> HHHHHHMFDVAKYLRRIGVEGTPPPTLDTLRHLHKRHLMAVPYDNSTAPDRLPASRHLTNVPLDLVFGHVVTEGHGGVCYELNRLFHTLLAELGYDVRMVAAAVRQANGTFGPEREHTFDLVHLDGRTHLVDVGFPGPSYSEPLYLSEEEQHQYGCSYRVTEHDGYRVVERRPKGSDWQPVYRFRPELADPSGWDAVRLLDSLDDYAQDSVLGTTFRSRATDNGKIVLIGRRYFTVEDGVERTKVLVKADEFQDVVDLILAGA

Amide synthases catalyze the formation of macrolactam rings from aniline-containing polyketide-derived seco-acids as found in the important class of ansamycin antibiotics. A key enzyme is the amide synthase ShGdmF (hereafter abbreviated as GdmF), which is not part of the PKS and is thought to catalyze the release of the ketide chain from the acyl carrier protein (ACP) domain of the last module 7 of the polyketide synthase. The overall folding of GdmF largely resembles the common architecture of its NAT analog, revealing a three-domain architecture with an N-terminal α-helical bundle (domain I, residues 1–88), a β-barrel (domain II, residues 89–185), and a C-terminal α/β-lid (domain III, residues 211–257), the latter being connected to domain II via an interdomain region (residues 186–210). The catalytic triad (Cys73-His111-Asp126 in GdmF) is highly conserved with an rmsd of 0.04 Å compared to the catalytic domain of MlNAT1 and is buried deep in the large active site cleft between domains II and III.

Crystals of ligand-free enzyme GdmF grew in rhombohedral form and diffracted to a resolution of 1.4 Å. Despite the low sequence identity of < 36%, the structural homology to prokaryotic and eukaryotic NATs is quite high for the refined GdmF structure with root mean square deviations (rmsd) of 1.5 Å for all backbone atoms compared to the structure of MlNAT1. As has been previously observed for prokaryotic NATs, and in contrast to eukaryotic NATs25, the C-terminal α/β-lid terminates in an α-helix positioned away from the deep active site cleft. The low crystallographic B-factors of the β-barrel and α/β-lid indicate fairly rigid domains with average values of 24 Å2. However, differences in the amino acid composition and their sidechain positions, particularly in residues 72 and 74, are found in close proximity to the catalytically important cysteine 73. This leads to a two- to threefold increased active site cleft with a volume of approximately 700 Å3 in GdmF. Despite the high resolution of the crystallographic data, there is no apparent electron density found for a major part of the interdomain region (residues 194–206), suggesting a highly flexible, mostly unstructured loop. In NAT structures, the interdomain region has a largely α-helical structure and closes the deep active site cleft and the catalytic triad. This altered loop region in GdmF appears to be a unique feature of amide synthases and contributes significantly to the widened active site cleft. Given that the native seco-substrate of GdmF is much larger, the wider active site cleft and flexible interdomain region may play a critical role in substrate binding and/or catalysis during macrolactamization.> GSHMTWLSDFPQAWAETGGMGLAVRQAPLIIPLKATSTPVSIKQYPMSQEARLGIKPHIQRLLDQGILVPCQSPWNTPLLPVKKPGTNDYRPVQDLREVNKRVEDIHPTVPNPYNLLSGLPPSHQWYTVLDLKDAFFCLRLHPTSQPLFAFE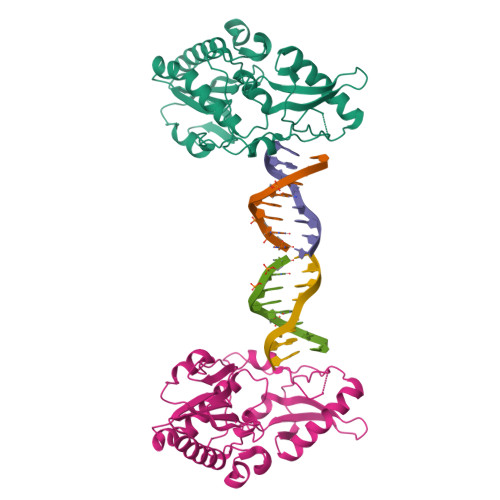WRDPEMGISGQLTWTRLPQGFKNSPTLFDEALHRDLADFRIQHPDLILLQYVDDLLLAATSELDCQQGTRALLQTLGNLGYRASAKKAQICQKQVKYLGYLLKEGQRLTRGSGC PACSIN/Syndapins are EFC (extended FCH (Fes/CIP4 homology)) domain proteins implicated in endocytosis because the C-terminal SH3 domain binds physically to the large GTPase dynamin, the phosphoinositide polyphosphatase synaptojanin, or the branched-actin regulator WASp. Consequently, it has been posited that PACSIN operates at the intersection between endocytosis and actin assembly. Drosophila Syndapin consists of an N-terminal membrane-binding EFC domain (residues 1–304) linked to a C-terminal SH3 domain (residues 439–494) by an unstructured linker including an EH domain-binding Asn-Pro-Phe (NPF) motif. We have solved the structure of the Drosophila Syndapin EFC domain (alternatively termed F-BAR due to the gross structural similarity of the EFC and BAR domains) that, together with the recent crystal structures of the human PACSIN 1 and -2 F-BAR domains, reveals unique features of this membrane-binding fold.

The structure of this domain (residues 14–301) was solved by X-ray crystallography at 2.7 Å resolution by single-wavelength anomalous dispersion (SAD). This EFC domain, like others that have been recently solved (FBP17/CIP4, FCHO2 and PACSIN), is a dimer resembling an elongated bowl when viewed from one side and a tilde-shape from another. Each monomer is composed of three long helices, designated α2 (residues 24–71), α3 (residues 76–118 and residues 127–172) and α4 (residues 182–190, 199–207, 213–253 and 261–273) that are flanked on one end by the N-terminal residues 14–23 and on the other by C-terminal residues 274–301, including a short C-terminal helix α5 (residues 277–288). Monomers dimerize in an antiparallel fashion to form a six-helical bundle core (α2–α4 from each monomer). The dimer interface is formed by residues restricted to helices α2 and α4. The insert in Drosophila Syndapin (120HHTLMQIK) is structured into a prong that protrudes approximately 18 Å from the concave face of the domain. Residues H121 to T122 and Q125 to I126 form two short β-strands hydrogen bonded into an antiparallel β-sheet scaffold, at the tip of which are positioned two hydrophobic residues, L123 and M124. This prong is surrounded by many basic residues that are also conserved in Syndapin homologues (K127, K130, H120, H121, R129, K28, K137, K35, K112). Yet the radius of curvature of the Syndapin EFC dimer (∼21 nm, assuming prong residues insert into the bilayer) is significantly smaller than CIP4 and FBP17 (both ∼30 nm) or FCHO2 (∼55 nm) making the packing angle of the Syndapin EFC dimer more similar to the radius of curvature of the N-BAR domains of amphiphysin and endophilin (both ∼11 nm) than to other EFC domains.

>[2x]SDSFWEPGNYKRTTKRIEDGYKLCNDLQQLIQERADIEKGYAKSLRTWSKKWGELIEKGPEYGTTEAAWKGVLTESERISDVHMKIKDNLCNDVNSQIKTWQKENYHHTLMQIKERKDLEDLFKKAQKPWAKLLAKVEKAKADYHSACKTERSATNQERNANADSSLSPDQVKKMHDRVQKTKDQVQKCREKYEQAIAEITKYNSVYIEDMTSVFEKCQTFEKTRLQFFKEILFNVHSCLDLTKVQSLPQIYEEFSHTINNADQQKDLKWWSNNHGINMAMNWPSFVEYT> GSHMAEEKWVVMVTAQTPTNIAVIKYWGKRDEVRILPINDSISVTLDPDHLCTLTTVAVSPSFDRDRMWLNGKEISLSGSRYQNCLREIRSRADDVEDKEKGIKIAKKDWEKLHLHIASHNNFPTAAGLASSAAGFACLVFALAKLMNVNEDPSQLSAIARQGSGSACRSLFGGFVKWNMGNKEDGSDSVAVQLVDDKHWDDLVIIIAVVSSRQKETSSTSGMRESVETSLLLQHRAKEVVPVRILQMEEAIKNRDFTSFTKLTCSDSNQFHAVCMDTSPPIFYMNDTSHRIISLVEKWNRSAGTPEIAYTFDAGPNAVMIARNRKVAVELLQGLLYCFPPKPDTDMKSYVLGDTSIVKEAGLEGELPQGIKDKIGSQDQKGEVSYFICSRPGRGPVVLQDQTQALLHPQTGLP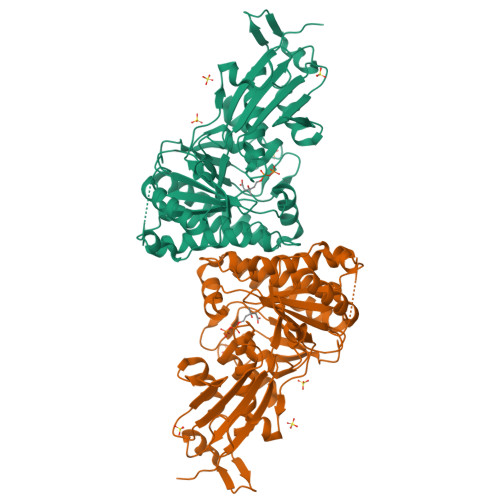K>[2x]EDGYDMWLRYQPIADQTL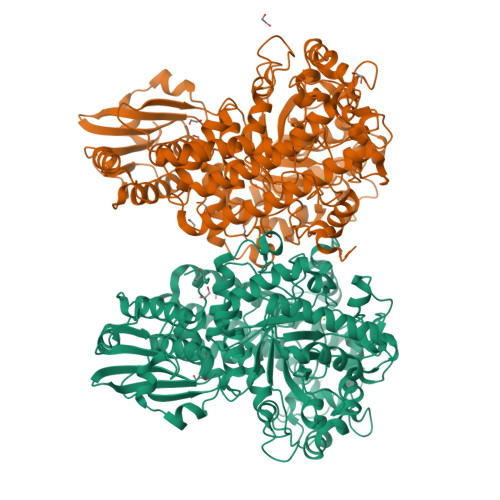LKTYQKQIRHLHVAGDSPTINAAAAELQRGLSGLLNKPIVARDEKLKDYSLVIGTPDNSPLIASLNLGERLQALGAEGYLLEQTRINKRHVVIVAANSDVGVLYGSFHLLRLIQTQHALEKLSLSSAPRLQHRVVNHWDNLNRVVERGYAGLSLWDWGSLPNYLAPRYTDYARINASLGINGTVINNVNADPRVLSDQFLQKIAALADAFRPYGIKMYLSINFNSPRAFGDVDTADPLDPRVQQWWKTRAQKIYSYIPDFGGFLVKADSEGQPGPQGYGRDHAEGANMLAAALKPFGGVVFWRAFVYHPDIEDRFRGAYDEFMPLDGKFADNVILQIKNGPIDFQPREPFSALFAGMSRTNMMMEFQITQEYFGFATHLAYQGPLFEESLKTETHARGEGSTIGNILEGKVFKTRHTGMAGVINPGTDRNWTGHPFVQSSWYAFGRMAWDHQISAATAADEWLRMTFSNQPAFIEPVKQMMLVSREAGVNYRSPLGLTHLYSQGDHYGPAPWTDDLPRADWTAVYYHRASKTGIGFNRTKTGSNALAQYPEPIAKAWGDLNSVPEDLILWFHHLSWDHRMQSGRNLWQELVHKYYQGVEQVRAMQRTWDQQEAYVDAARFAQVKALLQVQEREAVRWRNSCVLYFQSVAGRPIPANYEQPEHDLEYYKMLARTTYVPEPWHPASSSRVLK(2~{R})-1-[(2~{R})-1-[(2~{R})-1-(2-methoxyethoxy)propan-2-yl]oxypropan-2-yl]oxypropan-2-amine | C12 H27 N O4 | 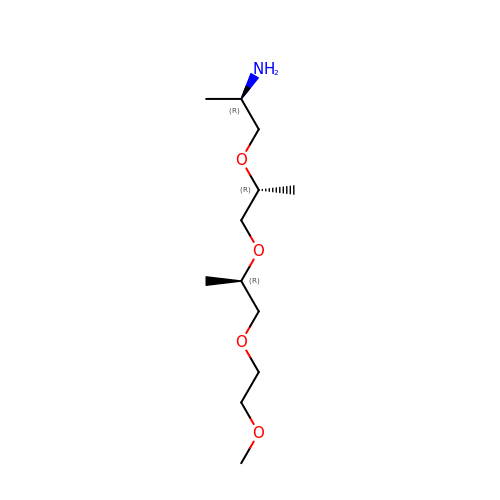JAVLCTSZYWYEEE-IJLUTSLNSA-N In the present study, we conducted structural and functional analyses of the heme-responsive sensor protein PefR (porphyrin-regulated efflux regulator) from the β-hemolytic bacterium Streptococcus agalactiae, which is the most common cause of life-threatening invasive bacterial infections (e.g., septicemia, pneumonia, and meningitis) during the neonatal period. Therefore, PefR promotes the expression of these heme efflux systems in S. agalactiae in response to the intracellular heme concentration, likely by binding heme. The monomer consists of six α-helices and two β-strands containing a winged helix-turn-helix (wHTH) motif. This architecture of PefR is similar to that of the multiple antibiotic resistance regulator (MarR) family of transcriptional regulators, in which helices α2–α4 and strands β1–β2 form the DNA-binding domains.

Indeed, in the apo-PefR–DNA complex structure, the α3–α4 helices of the wHTH regions of both subunits interact with the major grooves; in particular, the N-terminus of the α4 helix inserts into the major groove, and the wing (the loop between β1 and β2) inserts into the flanking AT-rich minor grooves of the target DNA. Lys63 and Ser64 in the α4 helix, and Arg89 in the wing, form hydrogen bonds with DNA bases (O atoms of G8, G18, and T6, respectively). Lys53 (in a loop on the edge of α3), Ser62 (in a loop between α3 and α4), Ser67 (α4), Arg72 (α4), and Lys75 (α4) apparently help stabilize the complex through hydrogen-bonding or electrostatic interactions with the phosphate backbones. Under the same conditions, the K53A, S62A, K63A, S67A, and K75A variants showed activity similar to that of wild-type PefR, and the R72A variant did not bind completely with the target DNA. These EMSA results suggested that the interaction between Arg89 and T6 in the minor groove is essential for target DNA association. In contrast, in the apo-PefR–DNA complex, there are direct hydrophobic interactions between these residues and there is no space to accommodate a heme. The Kd of H114A for DNA binding is 25 nM, similar to that of wild-type apo-PefR, clearly showing that His114 imidazole binding to the heme iron acts as a trigger for structural rearrangement. Given that the side chain of His114 faces the solvent region in the apo-PefR–DNA complex, free heme molecules might easily bind to His114, with His114 thus locking heme coordination. The distance between the Cα atom of Lys63 on the edge of the α4 helix (recognition helix for interaction with the major groove of DNA) and Arg89 in the wing loop of each subunit increased from 31 to 52 Å and from 54 to 76 Å, respectively. Given that the distance between two consecutive major grooves in B-DNA is ca. 34 Å, the increase in the interhelical distance between the recognition helices upon heme binding can promote the dissociation of holo-PefR from the target DNA.

>MENPLQKARILVNQLEKYLDRYAKEYDVEHLAGPQGHLVMHLYKHPDKDMSIKDAEEILHISKSVASNLVKRMEKNGFIAIVPSKTDKRVKYLYLTHLGKQKATQFEIFLEKLHSTMLAGITKEEIRTTKKVIRTLAKNMAMEDFDSLEVLFQ[2x]> TAELKICRVNRNSGSCLGGDEIFLLCDKVQKEDIEVYFTGPGWEARGSFSQADVHRQVAIVFRTPPYADPSLQAPVRVSMQLRRPSDREL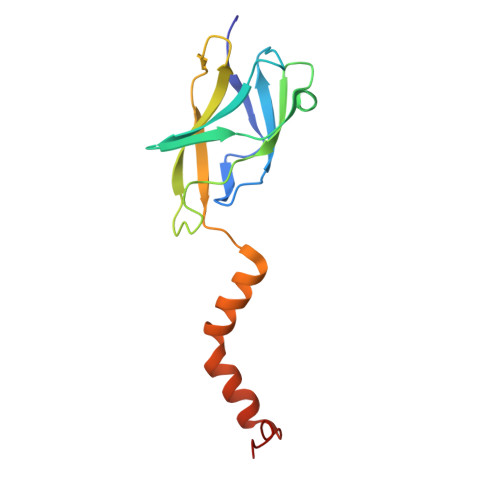SEPMEFQYLPDTDDRHRIEEKRKRTYETFKSIMKKSPFNGPTEPRP>KFESKAALLAARGPEELLCFTERLEDLVCFWEEAASAGVGPGNYSFSYQLEDEPWKLCRLHQAPTARGAVRFWCSLPTADTSSFVPLELRVTAASGAPRYHRVIHINEVVLLDAPVGLVARLADESGHVVLRWLPPPETPMTSHIRYEVDVSAGNGAGSVQRVEILEGRTECVLSNLRGRTRYTFAVRARMAEPSFGGFWS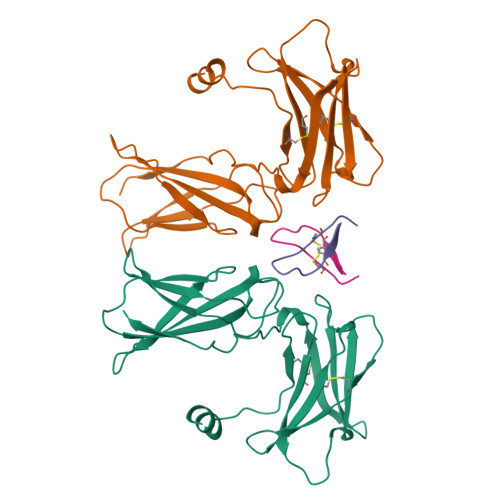AWSEPVSLLT[2x];>[2x]GGTYSCHFGPLTWVCKPQGG HAdV-D10 is a rare serotype isolated from the eyes of patients with conjunctivitis. HAdV are non-enveloped viruses measuring 90–100 nm and arranged in an icosahedral capsid with protruding fiber proteins at the pentameric vertices. Structural and biological studies of HAdV-D10 knob protein highlighted low-affinity engagement with native adenoviral receptors CAR and sialic acid. HAdV-D10 possesses characteristics of a promising virotherapy, combining low seroprevalence, weak receptor interactions, and reduced off-target uptake.

We produced a 2.5-Å crystal structure of HAdV-D10 fiber knob and modeled interactions with known viral receptors, and SPR was used to investigate binding of HAdV-D10 fiber knob with CAR, CD46, and DSG2. (A) 2.5-Å crystal structure of the HAdV-D10 fiber knob protein (HAdV-D10K). HAdV-D10 displayed weak but detectable binding to all three receptors. The highest-affinity interaction was with CAR. Predictive homology was used to model HAdV-D10K in complex with CAR, and the position of the DG loop interface indicated that HAdV-D10 can bind CAR, albeit at a lower affinity than HAdV-C5. Using recombinant HAdV-D10K protein, we confirmed binding to CAR in vitro with a 16.5-fold lower affinity than HAdV-C5K, as indicated by the IC50 values and demonstrated that CAR-binding HAdV-C5 recombinant knob blocks HAdV-C5/D10K infection. We conclude that, although the binding is weak, HAdV-D10 can bind and use CAR as an entry receptor. Although several binding sites were identified, we determined that HAdV-D10K forms weak interactions with CD46, insufficient for cell entry. We inserted A20 into the DG loop of HAdV-D10 fiber knob. Predictive models of HAdV-D10 fiber knob with A20 peptide depict the interaction with αvβ6 integrin.

>[12x]WNVKHDTRTLWTTPDTSPNCTIAQDKDSKLTLVLTKCGSQILANVSLIVVAGKYHIINNKNNPEIKSFTIKLLFDKNGVLLDNSNLGKTYWNFRSGDSNVSTAYEKAIGFMPNLVAYPKPSNSKKYARDIVYGTIYLGGKPDQPAVIKTTFNQETGCEYSITFDFSWSKTYENVEFETTSFTFSYIAQQ>GSSGSSGVQRLGASE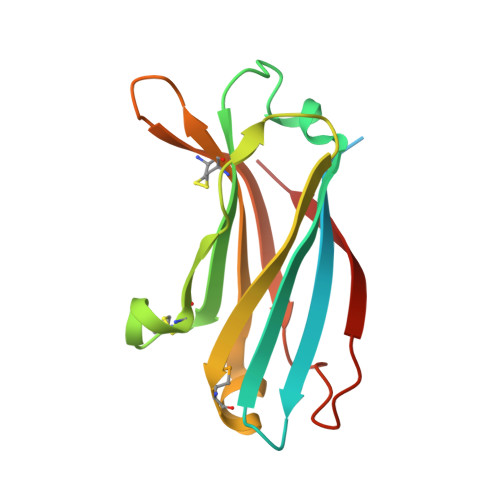AAAFDSDESEAVGATRIQIALKYDEKNKQFAILIIQLSNLSALLQQQDQKVNIRVAVLPCSESTTCLFRTRPLDASDTLVFNEVFWVSMSYPALHQKTLRVDVCTTDRSHLEECLGGAQISLAEVCRSGERSTRWYNLLS[2x]[(1S)-4-[hydroxy(methyl)amino]-1-(4-methylphenyl)-4-oxobutyl]phosphonic 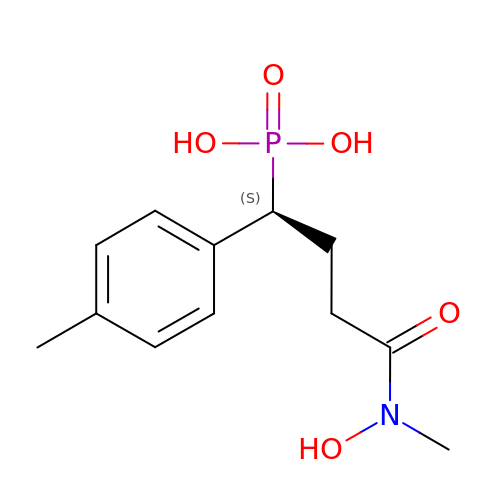acid | C12 H18 N O5 P | YBVPWURHYFIQDS-NSHDSACASA-N> MDMPVD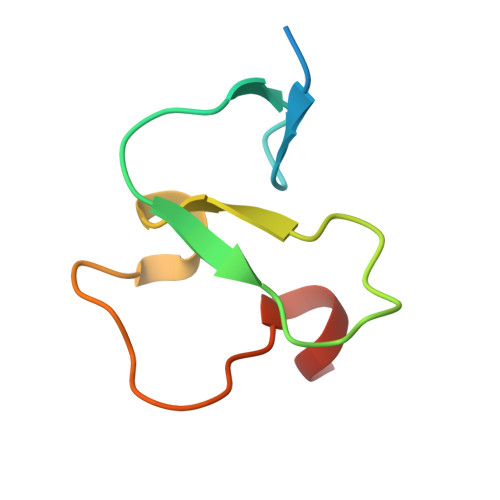PNEPTYCLCHQVSYGEMIGCDNPDCSIEWFHFACVGLTTKPRGKWFCPRCSQER Epoxomicin is a highly potent natural proteasome inhibitor and the structural scaffold for the anticancer drug carfilzomib. The biosynthesis of its α′,β′‐epoxyketone warhead involves the flavoenzyme EpxF, but a molecular understanding of the key catalytic reaction cascade remained elusive. In epoxomicin biosynthesis, this conversion is catalyzed by the flavoenzyme EpxF, which remains to be fully characterized. A high‐resolution crystal structure of EpxF revealed the architecture of the active site and enabled the identification of key catalytic residues.

Each subunit is composed of an N‐terminal α‐helical bundle, a seven‐stranded β‐sheet, and a C‐terminal α‐helical domain. Consistent with size exclusion chromatography data, EpxF assembles into a homodimer with an interface of approximately 2500 Å2, further stabilized by interactions between the C‐terminal loops of the monomers. The 2Fo‐Fc electron density map depicts FAD bound at two distinct catalytic centers located on opposite sides of the oxidoreductase. Notably, the substrate binding loop (residues 253–264) and a flexible region (residues 336–346) are not defined in the electron density map. The adenine moiety of each catalytic FAD is anchored within the dimeric interface, involving residues Ile301, Tyr309, Leu306, Glu490, Gln412, and Phe411. The phosphate groups are coordinated via hydrogen bonds to Arg299 and the peptide main chain atoms of residues 156 to 158. The isoalloxazine ring of FAD is planar, consistent with its oxidized quinoid state, and engaged in π‐stacking with Phe227. The C2 carbonyl is positioned in a pocket formed by residues 149–152, while the C4 carbonyl oxygen interacts with the backbone NH of Gly185, and N5 is aligned with the backbone of His183. Beyond these FAD interactions, our crystallographic analysis of EpxF revealed a well‐defined water molecule located 4.1 Å from Ser406, 3.3 Å from the Gly407 backbone amide, and 3.6 Å from the C4a atom of the flavin. This water molecule likely mimics the position of a C4a‐hydroperoxide and its geometry suggests that Ser406 may contribute to stabilizing such an intermediate.

> GSSIPGTTSFLEQLYVGRFRWDLIHPFPRQDEADRRVGDEVIAQLRQLIEDRVDPDVVDREARLPDGLVDELQKHGFLKARLGAEFGGLGLSHMNLFRLIEAAASWSVPVALVMAIENSVGVGPMHAHLPAGPLRDLVEARLRAGTVSGTADTEPAGAANHRRFTTATPTEDGTGYLLNGEKLHVGNAPIAEVLIVSASVVEDGVEHRRMFIVDTDSPGLRITARHEFMGVKGFPNGGMVFDNVFVPNERMVTNPPNDKARVTMEAVAMVIVGRLHMIVAPSLAIARQCLGWSREFVRARSIDGRPLGEYEEIQRRLAESAADVFAIEAIAEWSLLCPHWSDGINPWYEQSAAKNIGSVLGWRVAERTMSLLAGEGYETASSKSARGAARPFPLERALRDVRNFRISGGIDFQLDYWTSTIAIFTYYYPDPDNLAEIEANQVDLDSLVGSGLSERNERHLRHAAEQARKFSRLCRELSQRYPDLAALSEHERKLILIGQLSNELLAVALVLARAARLAGDGQDRAQALADVFCTGAGHRIADIWHQLAEEETPDYRSAAAADGN> MEFSGRKWRKLRLAGDQRNASYPHCLQFYLQPPSENISLIEFENLAIDRVKLLKSVENLGVSYVKGTEQYQSKLESELRKLKFSYRENLEDEYEPRRRDHISHFILRLAYCQSEELRRWFIQQEMDLLRFRFSILPKDKIQDFLKDSQLQFEAISDEEKTLREQEIVASSPSLSGLKLGFESIYKIPFADALDLFRGRKVYLEDGFAYVPLKDIVAIILNEFRAKLSKALALTARSLPAVQ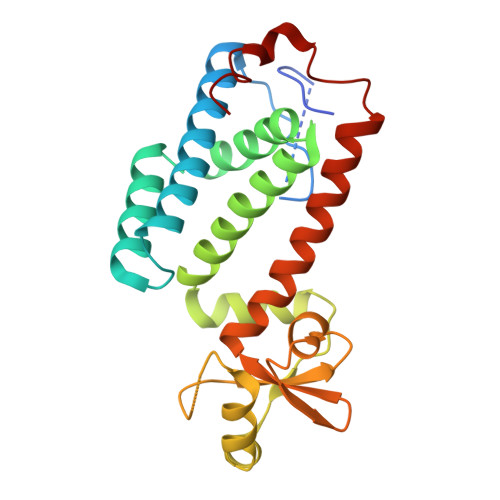SDERLQPLLNHL>[2x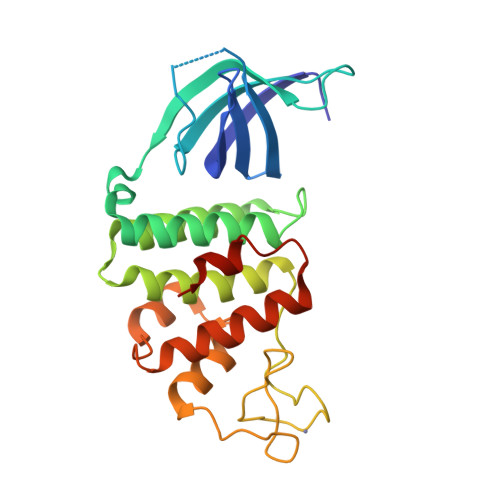]MRSRTANRSGIVIRRRVTPAGDIIVTLLTPQGKLKAIARGGVKGPLSSSLNLFHHVGVQVYQGPHNDLASVKQAVLEGALPTLAEPERYAFAHLMAEFADALFQEGEFSEQAFDLFAASLRGVAHQPDPEWVALVMSYKLLGLAGVIPQTARCARCGAPDPEHPDPLGGQLLCSKCAALPPYPPAVLDFLRHAVRRTVRASFEQPVPSADRPALWRALEKFVTVQVGGVHSWRQLVPSGVPVLS> GAMAEVQRYALVTGANKGIGFEICRQLAEKGIIVILTSRNEKRGLEARQKLLKELNVSENRLVFHQLDVTDLASVAAVAVFIKSKFGKLDILVNNAGVSGVEMVGDVSVFNEYIEADFKALQALEAGAKEEPPFKPKANGEMIEKFEGAKDCVVTNYYGPKRLTQALIPLLQLSPSPRIVNVSSSFGSLLLLWNEWAKGVLGDEDRLTEERVDEVVEVFLKDIKEGKLEESQWPPHFAAERVSKAALNAYTKIAAKKYPSFRINAICPGYAKTDITFHAGPLSVAEAAQVPVKLAL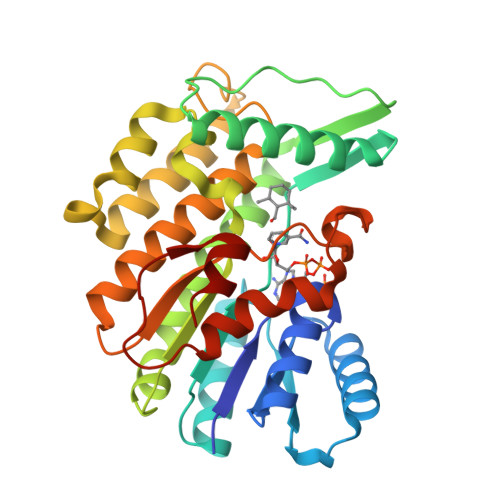LPDGGPSGCFFPRDKALALYLE>GSHMAAVQKLFPYTPRAPIRQGIYSQAVVVDRTMYISGQLGLDVASGKLVEGGVQAQARQALVNMGEILKAAGCGYDNVVKTTVLLADMNDFVNVNDVYKTFFSKNFPARA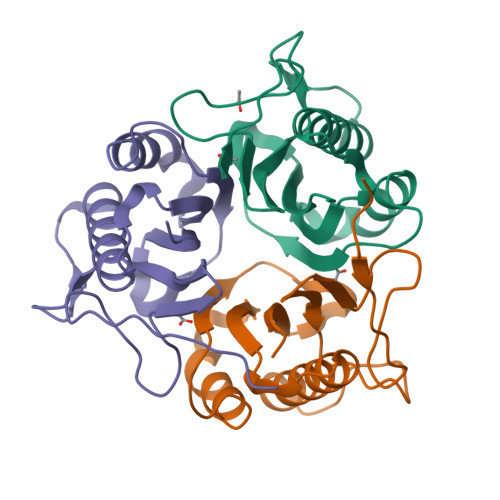AYQVVALPRGGLVEIEAVAVLGPISES[6x]>[2x]MLIAIEGVDGAGKRTLVEKLSGAFRAAGRSVATLAFP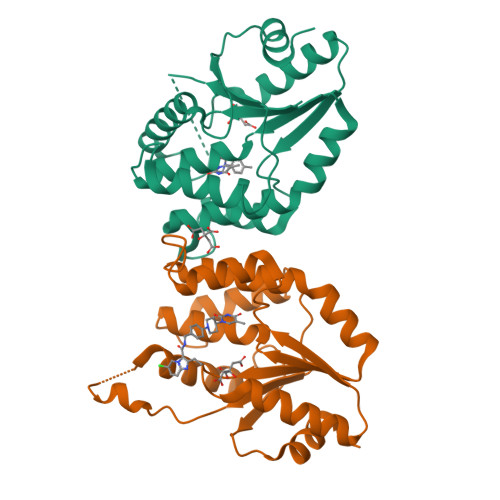RYGQSVAADIAAEALHGEHGDLASSVYAMATLFALDRAGAVHTIQGLCRGYDVVILDRYVASNAAYSAARLHENAAGKAAAWVQRIEFARLGLPKPDWQVLLAVSAELAGERSRGRAQRDPGRARDNYERDAELQQRTGAVYAELAAQGWGGRWLVVGADVDPGRLAATLAPPDVPS>MKEVTIEIKNKTGLHARP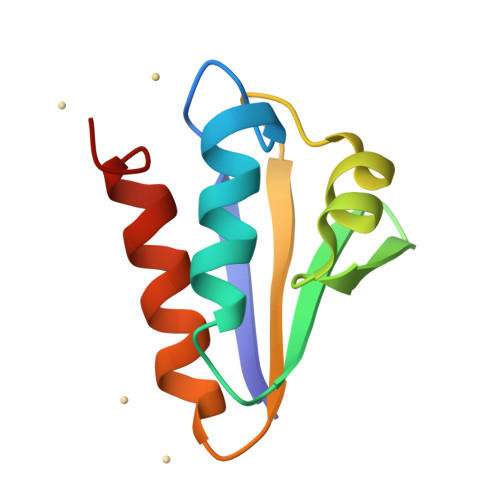AALFVQTASKFSSQIWVEKDNKKVNAKSIMGIMSLGVSQGNVVKLSAEGDDEEEAIKALVDLIESKFGEE[2x]>[37x]MALNSINTNSGALIALQNLNSTNAELTQVQQRINTGKKIGSAKDNGAIWATAKNQSATANSMNAVKDSLQRGQSTIDVALAAGDTITDLLGKMKEKALAASDTSLNTASFNALKSDFDSLRDQITKAASNAKFNGVSIANGSTAKLTFLANSDGSGFTVTAKTLTLTGLGLTASSTFTTAAAAKTMIGTIDTALQTA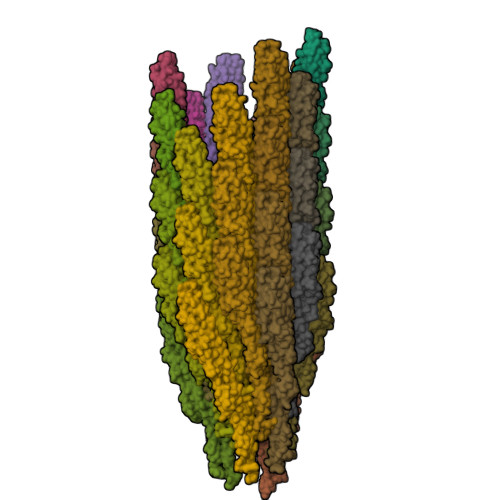TNKLASLGTSSTGLDTHLTFVGKLQDSLDAGVGNLVDADLAKESAKLQSLQTKQQLGVQALSIANSSSSAILSLFR>MKSRYLLFFLPLIVAKYTSAATMQPFHSPEESVNSQFYLPPPPGNDDPAFRYDKEAYFKGYAIKGSPRWKQAAEDADISVENIARIFSPVVGAKISPKDTPETWNMLQNLLKVGGYYATASAKKYYMRTRPFVLFNHSTCRPEDENTLRKDGSYPSGHTAYSTLLALVLSQARPERAQELARRGWEFGQSRVICGAHWQSDVDAGRYVGAVEFARLQTIPAFQKSLA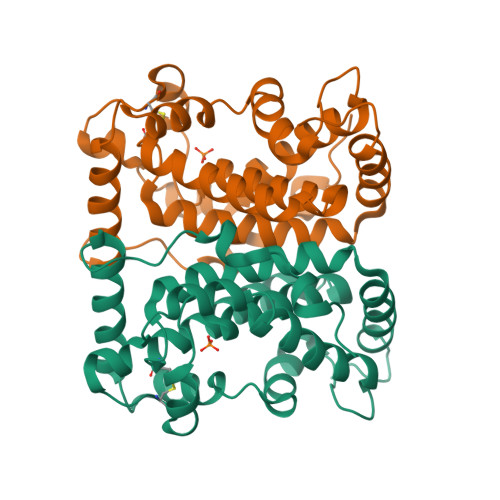KVREELNDKNNLLSKEERPELNY[4x]>[2x]SNASKSTKNDVKITALSTSESQIISHMLRLLIEHDTHGKIKPTLVNNLGSSTIQHNALINGDANISGVRYNGTDLTGALKEAPIKDPKKAMIATQQGFKKKFDQTFFDSYGFANTYAFMVTKE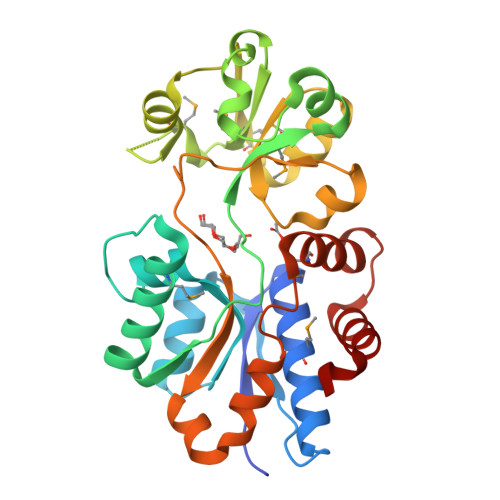TAKKYHLETVSDLAKHSKDLRLGMDSSWMNRKGDGYEGFKKEYGFDFGTVRPMQIGLVYDALNTEKLDVALGYSTDGRIAAYDLKVLKDDKQFFPPYAASAVATNELLRQHPELKTTINKLTGKISTSEMQRLNYEADGKGKEPAVVAEEFLKKHHYFD> MDTNDNAPKFERPSYEAELSENSPIGHSVIQ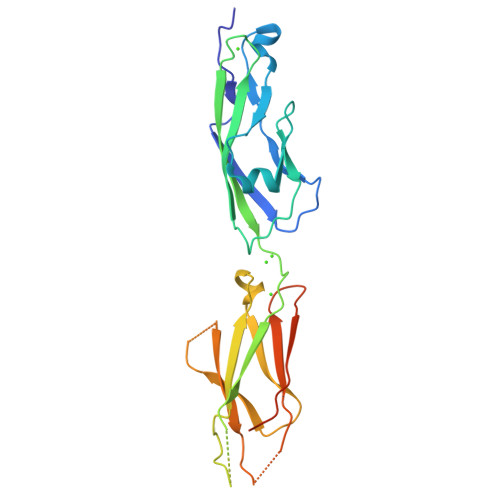VKANDSDQGANAEIEYTFHQAPEVVRRLLRLDRNTGLITVQGPVDREDLSTLRFSVLAKDRGTNPKSARAQVVVTVKDMNDNAPTIEIRGIGLVTHQDGMANISEDVAEETAVALVQVSDRDEGENAAVTCVVAGDVPFQLRQASETGSDSKKKYFLQTTTPLDYEKVKDYTIEIVAVDSGNPPLSSTNSLKVQVVDVNDNALEHHHHHH>MAWPGPLLLKDRKGRAYLVFPKEGGVFHHHKG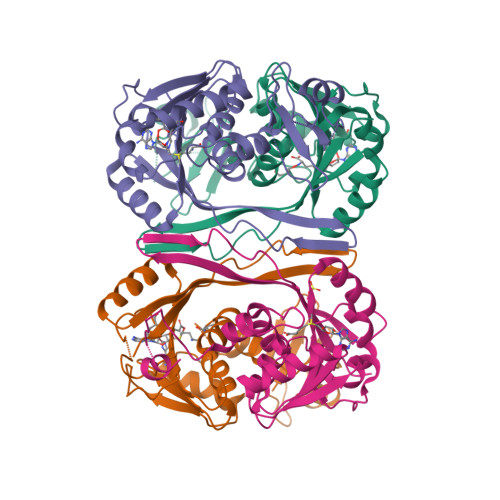SVPHEALLEAGPGGVVRTHLGEELSVHRPTLEEYLLHMKRSATPTAPKDASAMVTLLDLAPGMRVLEAGTGSGGLTLFLARAVGEKGLVESYEARPHHLAQAERNVRAFWQVENVRFHLGKLEEAELEEAAYDGVALDLMEPWKVLEKAALALKPDRFLVAYLPNITQVLELVRAAEAHPFRLERVLEVGWREWEVRLPVAHPRFQQVGHTAFLVALRRWKAS[4x]>[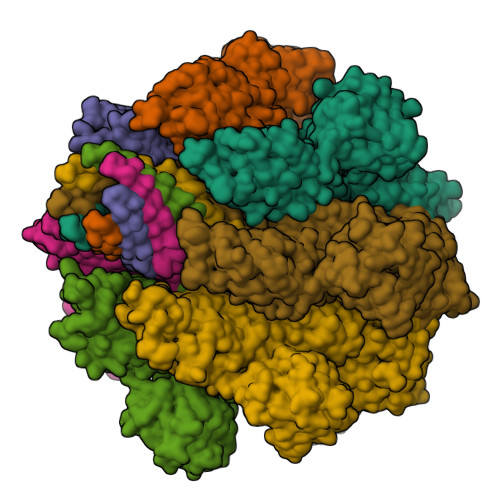7x]SGFASPAPANSETNTLPHVAFYISVNRAISDEECTFNNSWLWKNEKGSRPFCKDANISLIYRVNLERSLQYGIVGSATPDAKIVRISLDDDSTGAGIHLNDQLGYRQFGASYTTLDAYFREWSTDAIAQDYRFVFNASNNKAQILKTFPVDNINEKFERKEVSGFALGVTGGVEVSGDGPKAKLEARASYTQSRWLTYNTQDYRIERNAKNAQAVSFTWNRQQYATAESLLNRSTDALWVNTYPVDVNRISPLSYASFVPKMDVIYKASATETGSTDFIIDSSVNIRPIYNGAYKHYYVVGAHQFYHGFEDTPRRRITKSASFTVDWDHPVFTGGRPVNLQLASFNNRCIQVDAQGRLAANTCDSQQSAQSFIYDQLGRYVSASNTKLCLDGEALDALQPCNQNLTQRWEWRKGTDELTNVYSGESLGHDKQTGELGLYASSNDAVSLRTITAYTDVFNAQESSPILGYTQGKMNQQRVGQDHRLYVRAGAAIDALGSASDLLVGGNGGSLSSVDLSGVKSITATSGDFQYGGQQLVALTFTYQDGRQQTVGSKAYVTNAHEDRFDLPAAAKITQLKIWSDDWLVKGVQFDLN>GSHMTIKLIVGLANPGAEYAATRHNAGAWFVDLLAERLRAPLREEAKFFGYTSRVTLGGEDVRLLVPTTFMNLSGKAVAAMASFFRINPDEILVAHDELDLPPGVAKFKLGGGHGGHNGLKDIISKLGNNPNFHRLRIGIGHPGDKNKVVGFVLGKPPVSEQKLIDEAIDE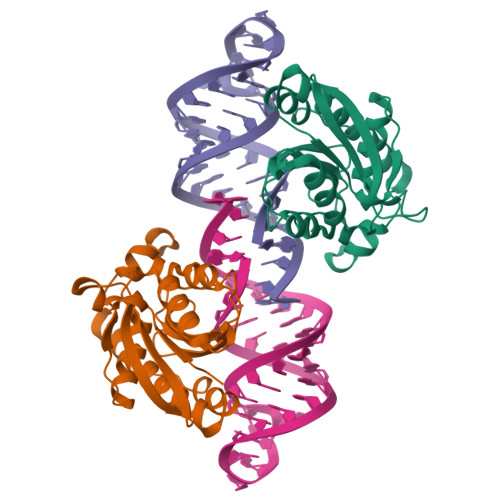AARCTEMWFTDGLTKATNRLHAFKAQ[2x]> MKHHHHHHHGAAGTSLYKKAGENLYFQGSMLPLYLLTNAKGQQMQIELKNGEIIQGILTNVDNWMNLTLSNVTEYSEESAINSE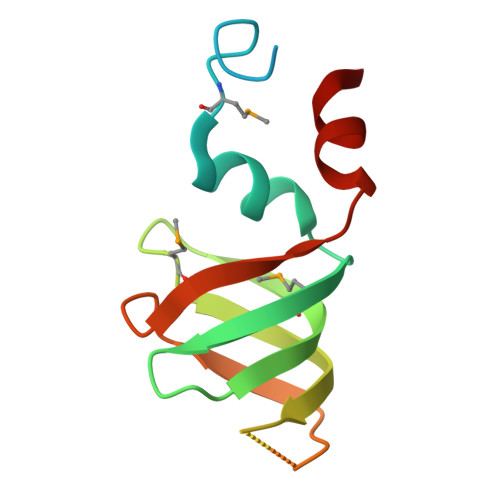DNAESSKAVKLNEIYIRGTFIKFIKLQDNIIDKVKQQI> SNAQESRLDRILESGVLRVATTGDYKPFSYRTEEGGYAGFDVDMAQRLAESLGAKLVVVPTSWPNLMRDFADDRFDIAMSGISINLERQRQAYFSIPYLRDGKTPITLCSEEARFQTLEQIDQPGVTAIVNPGGTNEKFARANLKKARILVHPDNVTIFQQIVDGKADLMMTDAIEARLQSRLHPELCAVHPQQPFDFAEKAYLLPRDEAFKRYVDQWLHIAEQSGLLRQRM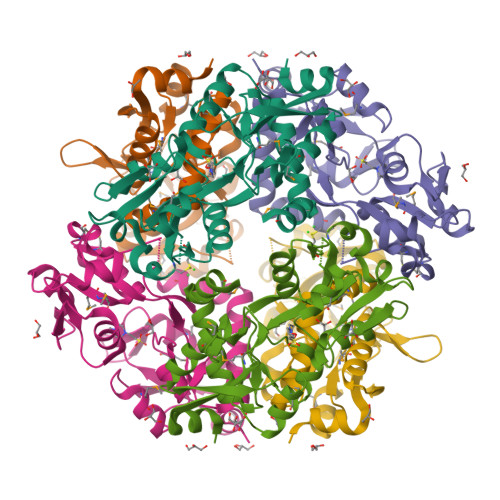EHWLEYR>MQSINFRTARGNLSEVLNNVEAGEEVEITRRGREPAVIVSKATFEAYKKAALDAE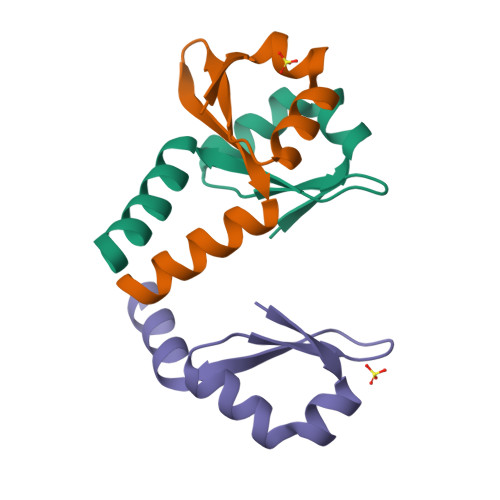FAS[8x]>GSRRASVGSHRFKVYNYMSPTFCDHCGSL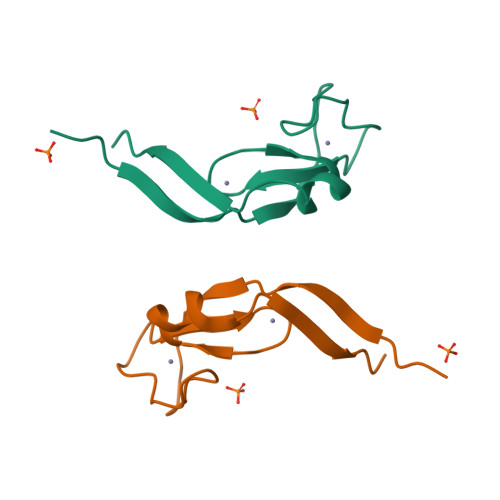LWGLVKQGLKCEDCGMNVHHKCREKVANLCEFIVTD[2x]>MSKLASECVANILNDWYIAIKQQDAESAERYFEEVKPLFDEMEEDQEVLMYYSLLEERHKMLLYQVKGEELPPHSYFNENHAEEIKKTDHMIEYYFFLFEALYESHKRNFEKAITLFKIAEKKLKDIPDCIERAEFYSKVA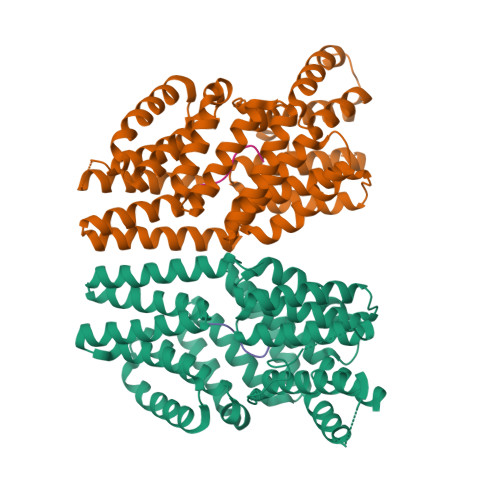SMYMMLRQSLISLNYINDSIQIYRENEGYKRKLATSLMIVGQNYTDLGLYEKAEESFLEAIRISRVLHDSLFTALIHHNLSITYSAANRSQDCINALKKAIRNKEWRDSVYYINSLYMFLKELYKIGDVNKMPYYYKKTKEYFKRKENKVYEAKINIIYGLLQQDQRKSIETCRGGISYLYEVNDLDSVFDLSLVISEHCEKHGLYKEALEFSKHAILAEEKMRHLEGL[2x];>ERPVGT[2x]> MLLRRATRLARVYGGGATTAFVPGSSSSSSSSSSTASVGADYLRGRSIGAKALLGRRARQGSLFAVAN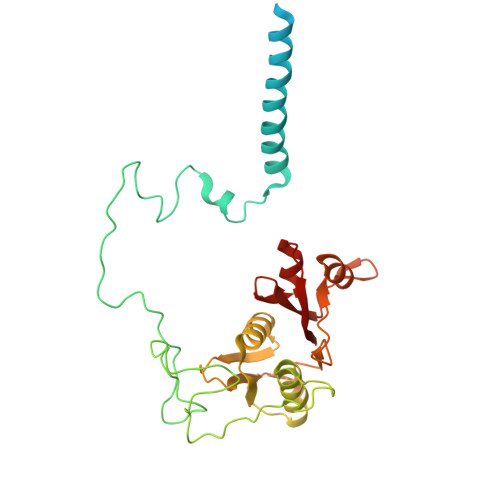DVTVSEKRVRQQLNALLADERDPLAEARRQSSAAEGFASSARPFPQRPLVNLPGVERVRDLPADPITRLFFQHQGDHALYYGTYDEPSRLDEDRVQLEKREPKDWTFNVFTPVYDFCHRLREASEQRKRFVIVPSTIETRGCAKVLLDHGLVAGFRDFRNDRAFAVELKYFQNEPTINIIEPCSYDGKTEFEWSPKMMRRLMNAHGIHNRLIIYICRTADNRIIDHIQAVKECIGGRGLMMAH> MQREEKQLEASLDALLNQVADLKNSLGSFIYKLENEYDRLTWPSVLDSFALLSGQLNTLNKVLKHEKTPLFRNQVIIPLVLSPDRDEDLMRQTEGRVPVFSHEVVPDHLRTKPDPEVEEQEKQLTTDAARIGADAAQKQIQSLNKMCSNLLEKISKEERESESGGLRPNKQTFNPGDTNALVAAVAFGKGLSN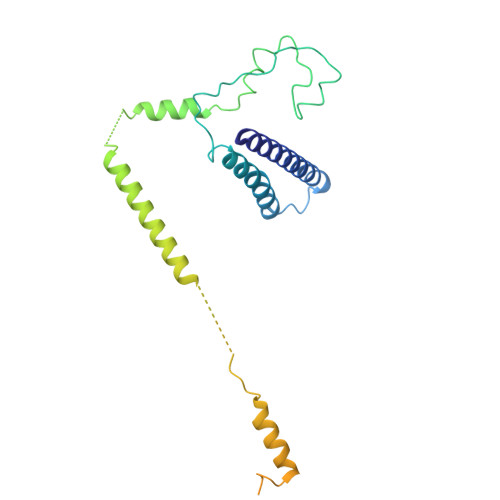WRPSGSSGPGQPGQPGAGTILAGASGLPQVQMPGAPNQQQPMLSGVQMAQAGQPGKMPSGIKTNIKSASMHPYQR>ADKLFINALKKKFEESPEEKKTTFYTLGGWKQSERKTEFVNAGKEVAAKRGIPQYNPDIGTPLGQRVLMPYQVSTTDTYVEGDDLHFVNNAAMQQMWDDIRRTVIVGLNHAHAVIEKRLGKEVTPETITHYLETVNHAMPGAAVVQEHMVETHPALVADSYVKVFTGNDEIADEIDPAFVIDINKQFPEDQAETLKAEVGDGIWQVVRIPTIVSRTCDGATTSRWSAMQIGMSMISAYKQAAGEAATGDFAYAAKHAEVIHMGTYLPVRRARGENEPGGVPFGYLADICQSSRVNYEDPVRVSLDVVATGAMLYDQIWLGSYMSGGVGFTQYATAAYTDNILDDFTYFGKEYVEDKYGLCEAPNNMDTVLDVATEVTFYGLEQYEEYPALLEDQFGGSQRAAVVAAAAGCSTAFATGNAQTGLSGWYLSMYLHKEQHSRLGFYGYDLQDQCGASNVFSIRGDEGLPLELRGPNYPNYAMNVGHQGEYAGISQAPHAARGDAFVFNPLVKIAFADDNLVFDFTNVRGEFAKGALREFEPAGERALITPAK[2x];>AKFEDKVDLYDDRGNLVEEQVPLEALSPLRNPAIKSIVQGIKRTVAVNLEGIENALKTAKVGGPACKIMGRELDLDIVGNAESIAAAAKEMIQVTEDDDTNVELLGGGKRALVQVPSARFDVAAEYSAAPLVTATAFVQAIINEFDVSMYDANMVKAAVLGRYPQSVEYMGANIATMLDIPQKLEGPGYALRNIMVNHVVAATLKNTLQAAALSTILEQTAMFEMGDAVGAFERMHLLGLAYQGMNADNLVFDLVKANGKEGTVGSVIADLVERALEDGVIKVEKELTDYKVYGTDDLAMWNAYAAAGLMAATMVNQGAARAAQGVSSTLLYYNDLIEFETGLPSVDFGKVEGTAVGFSFFSHSIYGGGGPGIFNGNHIVTRHSKGFAIPCVAAAMALDAGTQMFSPEATSGLIKEVFSQVDEFREPLKYVVEAAAEIKNEI[2x];>AQYYPGTTKVAQNRRNFCNPEYELEKLREISDEDVVKILGHRAPGEEYPSVHPPLEEMDEPEDAIREMVEPIDGAKAGDRVRYIQFTDSMYFAPAQPYVRSRAYLCRYRGADAGTLSGRQIIETRERDLEKISKELLETEFFDPARSGVRGKSVHGHSLRLDEDGMMFDMLRRQIYNKDTGRVEMVKNQ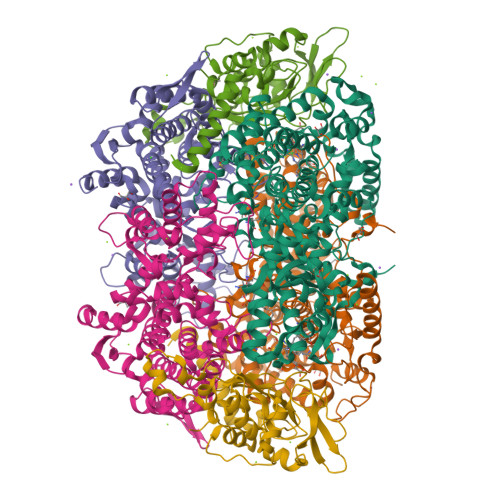IGDELDEPVDLGEPLDEETLMEKTTIYRVDGEAYRDDVEAVEIMQRIHVLRSQGGFNLE[2x]> GGGSGGGS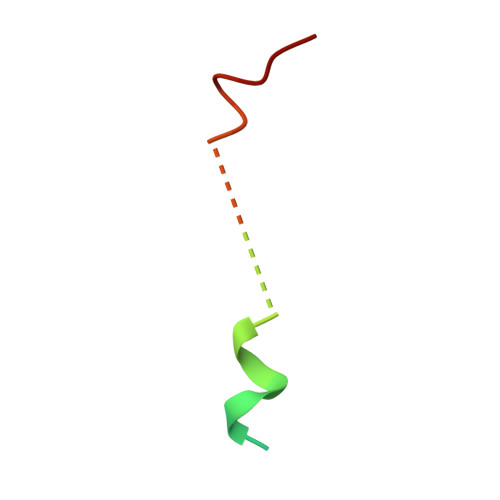KKHSLDLLSKERELNGKLRHLSP>[4x]ATDRGSESDKHFRKVSDKEKIDQLQEELLHTQLKYQRILERLEKENKELRKLVLQKDDKGIHHRKLKKSLIDMYSEVLDVLSDYDASYNTQDHLPRVVVVGDQSAGKTSVLEMIAQARIFPRGSGEMMTRSPVKVTLSEGPHHVALFKDSSREFDLTKEEDLAALRHEIELRMRKNVKEGCTVSPETISLNVKGPGLQRMVLVDLPGVINTVTSGMAPDTKETIFSISKAYMQNPNAIILCIQDGSVDAERSIVTDLVSQMDPHGRRTIFVLTKVDLAEKNVASPSRIQQIIEGKLFPMKALGYFAVVTGKGNSSESIEAIREYEEEFFQNSKLLKTSMLKAHQVTTRNLSLA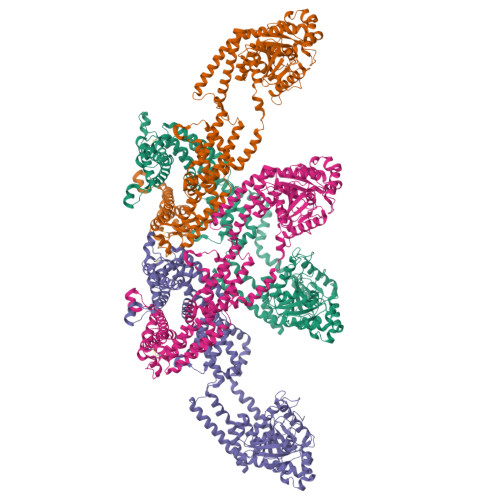VSDCFWKMVRESVEQQADSFKATRFNLETEWKNNYPRLRELDRNELFEKAKNEILDEVISLSQVTPKHWEEILQQSLWERVSTHVIENIYLPAAQTMNSGTFNTTVDIKLKQWTDKQLPNKAVEVAWETLQEEFSRFMTEPKGKEHDDIFDKLKEAVKEESIKRHKWNDFAEDSLRVIQHNALEDRSISDKQQWDAAIYFMEEALQARLKDTENAIENMVGPDWKKRWLYWKNRTQEQCVHNETKNELEKMLKCNEEHPAYLASDEITTVRKNLESRGVEVDPSLIKDTWHQVYRRHFLKTALNHCNLCRRGFYYYQRHFVDSELECNDVVLFWRIQRMLAITANTLRQQLTNTEVRRLEKNVKEVLEDFAEDGEKKIKLLTGKRVQLAEDLKKVREIQEKLDAFIEALHQEK> SNAAQISDGKQYITLDKPVAGEPQVLEFFSFY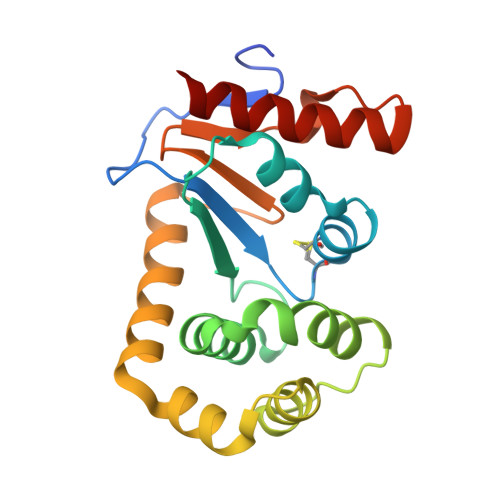CPHCYQFEEVLHVSDNVKKKLPEGTKMTKYHVEFLGPLGKELTQAWAVAMALGVEDKVTVPLFEAVQKTQTVQSAADIRKVFVDAGVKGEDYDAAWNSFVVKSLVAQQEKAAADLQLQGVPAMFVNGKYQINPQGMDTSSMDVFVQQYADTVKYLVDKK> SLMVEKPQLKFKSPIDNSESHPFIPLLKEKPNALKPLSESLRLVDDDENNPSHYPHPYEYEIDHQEYSPEILQIREEIPSKSWDDSVPIWVDTSTELESMLEDLKNTKEIAVNLEHHDYRSYYGIVCLMQISTRERDYLVDTLKLRENLHILNEVFTNPSIVKVFHGAFMDIIWLQRDLGLYVVGLFDTYHASKAIGLPRHSLAYLLENFANFKTSKKYQLADWRIRPLSKPMTAYARADTHFLLNIYDQLRNKLIESNKLAGVLYESRNVAKRRFEYSKYRPLTPSSEVYSPIEKESPWKILMYQYNIPPEREVLVRELYQWRDLIARRDDESPRFVMPNQLLAALVAYTPTDVIGVVSLTNGVTEHVRQNAK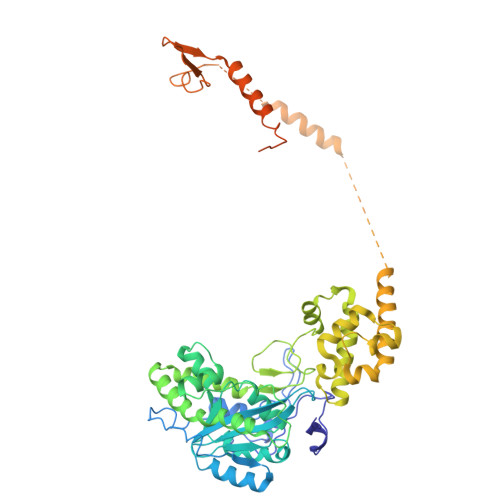LLANLIRDALRNIKNTNEEATPIPSSETKADGILLETISVPQIRDVMERFSVLCNSNISKSRAKPVTNSSILLGKILPREEHDIAYSKDGLPNKVKTEDIRIRAQNFKSALANLEDIIFEIEKPLVVPVKLEEIKTVDPASAPNHSPEIDNLDDLVVLKKKNIQKKQPAKEKGVTEKDAVDYSKI> PVELTIATFNEFGYSDLYREYEAAHPNVKITERRAATVDEHIKNLETNLASGSGMADIEAMEVSWIYKYLAKADKFVDLRDHGADELKSRWLDWKVASATTSDGRIIGYGTDI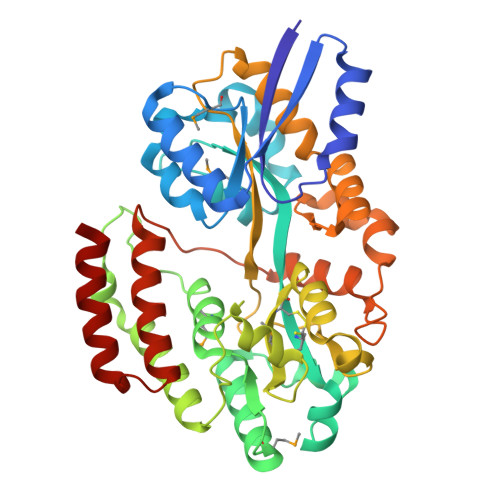GPEAICYRRDLFARAGLPTDRAEVAKLFPDWTSYFAAGRRFKAKMPNSAWFDSAVLTWEAMRNQLIQAYYSNQDRYLGDENELLKRTWDQIVAATEDGLSAKLPAWSDAWTKAFRTDAFATMACPGWLLGVIADNAGTFGKGKWDVADVFPGGGGNWGGSYLTVPTQSTQPAEAAKLAAWLTAPEQQIKVFKKVGSFPSTVDAYESEQVTAQVNPYFNNAPVGKIFVNRANNVILKQHKGPRDGEINQVFTEALARVDEGKQSSSAAWKQALREADKAAN>[2x]SNAMLSINPNEQTEKDNYKLLTGSIIPRPVAFVTSVTKEGVLNGAPYSYFNIVAANPPLISVSVQR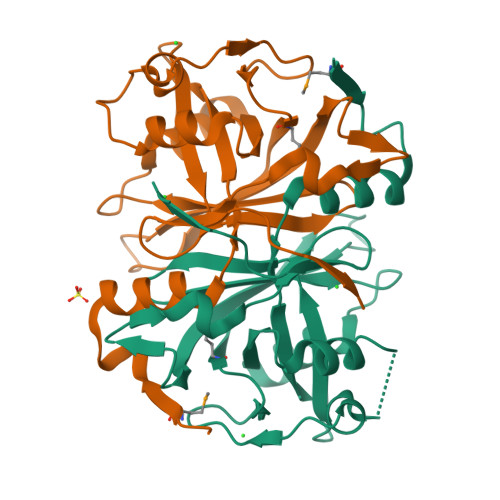KAGERKDTSRNAIEKGEFVVHISDESYVAAINETAANLPPNESEIELAKLTPIESEVISVPGVKEANIRMECVLERAIPLGGTEDSPACDLLIGRVVRFHVAEHLYEKGRIHAEGLKPISRLAGHNYAKLGEQFELVRPI>[2x]GHMSTTARADSIGGLFEDFTQSAAQRAIEVRTIFHMIGDVSGKSVLDLACGFGFFGREIYRRGAAKVVGVDISEKMIELAREE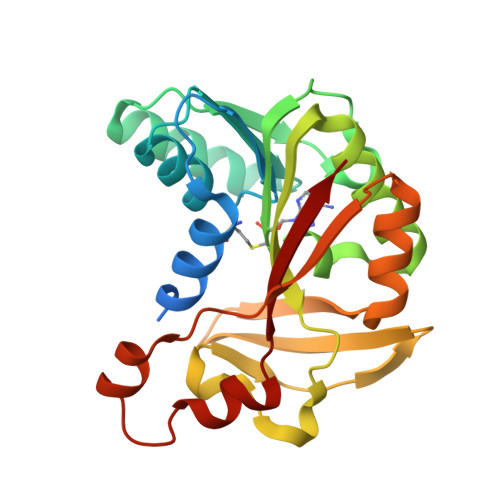SRKYGDPLEFHVRDVANMEPLGQFDLVNAAWLFNYADSVENLRKMFKVVRASLKPDGKLVAYTVDPDFSLAKGNFAKYGVNVLNERAWGPGYRHDAEFVTDPPSQFSFYRWSRADYESAIADAGFSHFEWQKPLLEADDIATHPPGFWDVFQNNCLQTGLVCKP> KKKRGKKEKVILNAEQVATKTRLPPIRLEDRITPEPPATVARNIRSQISRAVAGWKTKRMFTYRNKYRLRRLVGMTHDIDSDDEFAQANARTRETNASTSKVSSSGCSTEKAEGVNGSTMGRRNRPSFAGRTFVTPLTKLQHQAALPRSPLHARFDFPHTVHYDVFWGPPQVEEEPNKSGCWVSFRVADLKL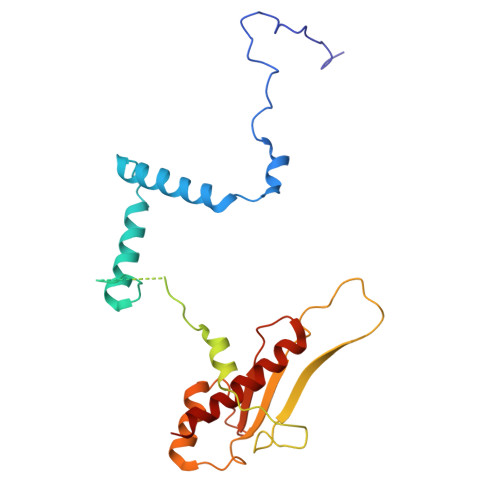SDSQEQRLLDILGPERYDEQTGVVCLEADVFPQLNHNAAYLGDILQQLMREVKK>[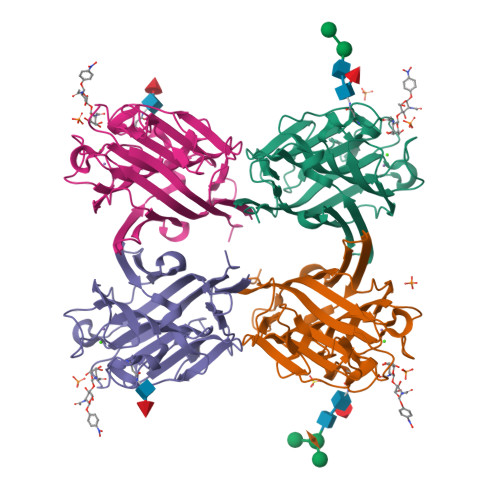4x]KETTSFVFTRFSPDPQNLLLQGDTVVTSSGHLQLTQVKDGEPVYSSLGRALYYAPIHIWDSNTDTVANFVTSFSFVIDAPNKAKAADGLAFFLAPVDTEPQKPGGLLGLFHDDRHNKSNHIVAVEFDTFKNSWDPEGTHIGINVNSIVSRKTISWDLENDEVANVVISYQASTKTLTASLVYPSSSTSYILNDVVDLKQILPEYVRVGFTAASGLSKDHVETHDVLAWTFDSDLPDPSSDDCN> SALVETRTIVRF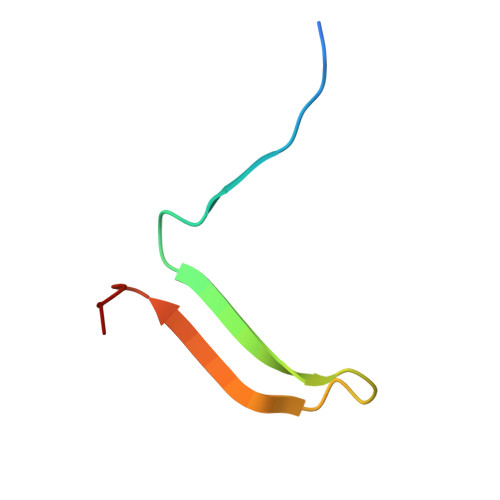NRPFLMIIVDHFTWNIFFMSKVTNPKQA Glycolyl-CoA carboxylase (GCC) is a new-to-nature enzyme that catalyzes the key reaction in the tartronyl-CoA (TaCo) pathway, a synthetic photorespiration bypass that was recently designed to improve photosynthetic CO2 fixation. GCC was created from propionyl-CoA carboxylase (PCC) through five mutations. The enzyme forms an α6β6 dodecameric complex, where the β-subunits arrange in a central core of two trimeric layers, while the α-subunits sit on top of the core and face outward. The biotin cofactor that is essential to catalysis is covalently linked to a lysine residue in the BCCP domain of the α-subunit and acts as a flexible arm that transfers the carboxyl group derived from HCO3– between the active sites of the α- and β-subunits.

Besides G20R, we also identified variant L100N that showed a significantly decreased ATP to carboxylation ratio of 1.7 ± 0.1 ATP, lowering the energy demand for the reaction by 60% compared to GCC M5 (4.0 ± 0.0 ATP per glycolyl-CoA carboxylation). In this variant, Leu100 in the active site periphery (second shell) was replaced by Asn. To identify structural changes that might be responsible for the catalytic improvements of the G20R or L100N variants, we solved their cryo-EM structures at 2.05 and 2.31 Å, respectively. The L100N substitution is located in the periphery of the active site, at a position that had previously been targeted during engineering efforts of GCC M5, in which this position was engineered to be serine. The Asn100 substitution is in close proximity to His143, which was proposed to coordinate the hydroxyl group of glycolyl-CoA. While active site overlays of the L100N variant and GCC M5 look almost identical, we assume that Asn100 forces His143 into a more favorable rotamer conformation for substrate binding and catalysis, enabling carboxylation to occur more efficiently. This is supported by the fact that His143 is categorized as a rotamer outlier in all subunits of the L100N cryo-EM structure, which is not the case for the GCC M5 or G20R variant structures. While the L100N variant exhibits a slightly increased proportion of higher mass oligomeric complexes in MP experiments, the complex distribution remained similar to that of GCC M5 and PCC.

>[6x]MKDILEKLEERRAQARLGGGEKRLEAQHKRGKLTARERIELLLDHGSFEEFDMFVQHRSTDFGMEKQKIPGDGVVTGWGTVNGRTVFLFSKDFTVFGGSNSEAHAAKIVKVQDMALKMRAPIIGIFDAGGARIQEGVAALGGHGEVFRRNVAASGVIPQISVIMGPCAGGDVYSPAMTDFIFMVRDTSYMFVTGPDVVKTVTNEVVTAEELGGAKVHTSKSSIADGSFENDVEAILQIRRLLDFLPANNIEGVPEIESFDDVNRLDKSLDTLIPDNPNKPYDMGELIRRVVDEGDFFEIQAAYARNIITGFGRVEGRTVGFVANQPLVLAGVLDSDASRKAARFVRFCNAFSIPIVTFVDVPGFLPGTAQEYGGLIKHGAKLLFAYSQATVPLVTIITRKAFGGAYIVMASKHVGADLNYAWPTAQIAVMGAKGAVEIIFRAEIGDADKVAERTKEYEDRFLSPFVAAERGYIDEVIMPHSTRKRIARALGMLRTKEMEQPRKKHDNIPL;>[6x]MFDKILIANRGEIACRIIKTAQKMGIKTVAVYSDADRDAVHVAMADEAVHIGPAPAAQSYLLIEKIIDACKQTGAQAVHPGYGFLSERESFPKALAEAGIVFIGPNPGAIAAMGDKIESKKAAAAAEVSTVPGFLGVIESPEHAVTIADEIGYPVMIKASAGGGGKGMRIAESADEVAEGFARAKSEASSSFGDDRVFVEKFITDPRHIEIQVIGDKHGNVIYLGERECSIQRRNQKVIEEAPSPLLDEETRRKMGEQAVALAKAVNYDSAGTVEFVAGQDKSFYFLEMNTRLQVEHPVTEMITGLDLVELMIRVAAGEKLPLSQDQVKLDGWAVESRVYAEDPTRNFLPSIGRLTTYQPPEEGPLGGAIVRNDTGVEEGGEIAIHYDPMIAKLVTWAPTRLEAIEAQATALDAFAIEGIRHNIPFLATLMAHPRWRDGRLSTGFIKEEFPEGFIAPEPEGPVAHRLAAVAAAIDHKLNIRKRGISGQMRDPSLLTFQRERVVVLSGQRFNVTVDPDGDDLLVTFDDGTTAPVRSAWRPGAPVWSGTVGDQSVAIQVRPLLNGVFLQHAGAAAEARVFTRREAELADLMPVKENAGSGKQLLCPMPGLVKQIMVSEGQEVKNGEPLAIVEAMKMENVLRAERDGTISKIAAKEGDSLAVDAVILEFA> LPPTEQDLT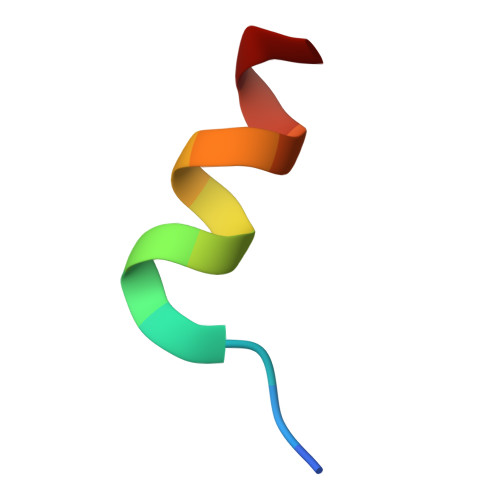KLLLE> AMNYFVGNSLGVNLTGIEKAIINRLNLFKEMGRPAQCVFLSWNRYLYRNAQNYITS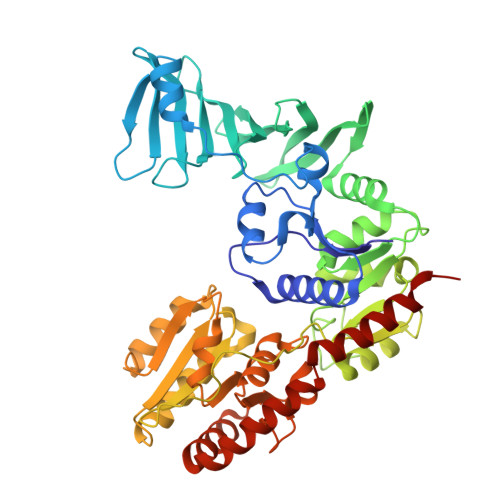SDYINMYDFFQEATYLERNEPFDWLSYWTDECHYTLKHVENSHDFRIYDQERFLMYAHFQDPKYRILDYVNHFDSQRRKVKRDFYDVRGFLSCSRILVDKQQTLCEFFYNPEGDTKLEKYFSYKDGKPEVQKIIVYYANKQYFFNNETELGAFFIKQLYQHGDLFFSDRNVYTAPIFNLTPESIPVVAVLHSTHIKNIDALDSSPFKNVYKAMFENLSRYRAIIVSTEQQKLDVEKRINHTIPVVNIPVGYSETIDTPVQTLDQRSVKLISVARYSPEKQLHQQIELIKRLVSYVPKIELHMYGFGSESKKLNELIQKYGLENHVYLRGFLSNLDQEYSDAYLSLITSNMEGFSLALLESLAHGVPVISYDIKYGPNELITSDFNGYLITKNDEDALFDKVKYVIDHPEVQQRLSKGSLAKAQQYSKASLIKQWDQFVRLILEHHHHHH>MTEAQAIAKQLGGVKPDDEWLQAEIARLKGKSIVPLQQVKTLHDWLDGKRKARKSCRVVGESRTGKTVACDAYRYRHKPQQEAGRPPTVPVVYIRPHQKCGPKDLFKKITEYLKYRVTKGTVSDFRDRTIEVLKGCGVEMLIIDEADRLKPETFADVRDIAEDLGIAVVLVGTDRLDAVIKRDEQVLERFRAHLRFGKLSGEDFKNTVEMWEQMVLKLPVSSNLKSKEMLRILTSATEGYIGRLDEILREAAIRSLSRGLKKIDKAVLQEVAKEYK[11x];>MIEAPDVKPWLFLIKPYEGESLSHFLGRFRRANHLSASGLGTLAGIGAIVARWER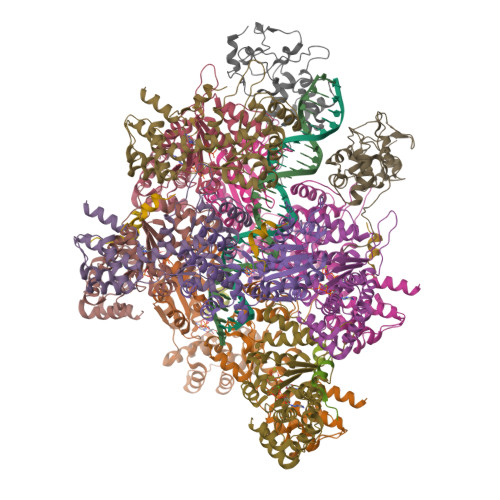FHFNPRPSQQELEAIASVVEVDAQRLAQMLPPAGVGMQHEPIRLCGACYAESPCHRIEWQYKSVWKCDRHQLKILAKCPNCQAPFKMPALWEDGCCHRCRMPFAEMAKLQKV[2x];>[9x]IEVWDYEQLREEYGF3-[(3R)-3-ethyl-1-{9-[(3S)-3-ethyl-3-(3-hydroxyphenyl)azepan-1-yl]nonyl}azepan-3-yl]phenol | C37 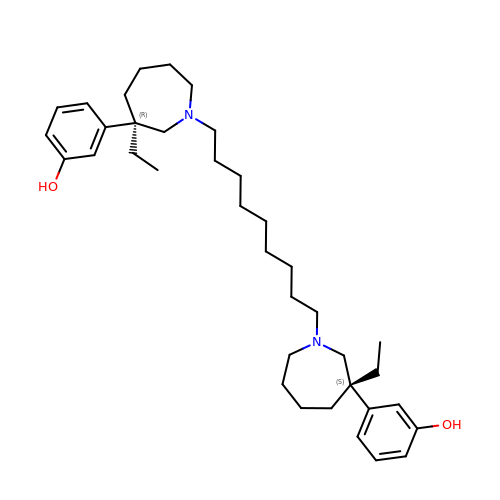H58 N2 O2 | ZZKZUUMHRSWLQQ-JXLNJXQWSA-N>MGGEIITLQAGQCGNHVGKFLWSQLAKEHAIGTDGLSQLPDSSTERDDDTKPFFRENSRNKFTPRAIMMDSEPSVIADVENTFRGFFDPRNTWVASDGASAGNSWANGYDIGTRNQDDILNKIDKEIDSTDNFEGFQLLHSVAGGTGSGLGSNLLEALCDRYPKKILTTYSVFPARSSEVVVQSYNTILALRRLIEDSDATVVFDNASLLNISGKVFRNPNIDLQHTNQLISTIISSVTNSIRFPSYMYSSMSSIYSTLIPSPELHFLSPSFTPFTSDYIHDDIAHKGHSSYDVMLDLLDPSNSLVSTAMNNPTYFNVYNTIIGNVEPRQISRAMTKLQQRIKFPSWSSSAMHVNIGRRSPYLPLQPNENEVSGMMLSNMSTVVNVFENACNTFDKVFAKGAFLNNYNVGDLFQSMQNVQDEFAESREVVQSLMEDYVAAEQDSYLDDVLVDDENMVGELEEDLDADGDHKLV[2x];> MEIKEVDDRAELLRYTNNIPLLGKLVNHQPLWSTNPKLKSFSLEKISAPDQRRVQEALVVKDLLNVLIGLEGTYIRYFNDYEPSDPETPIEFKIAKKMDPSFKTFSRRIVRYGKQYMILTRAYEKWSDTSFGMVLQRFAYEIRRFLEDVYLKTLVERLERDFNKVPNFSIRELEQIINETEVNKQMELLYNIYEEIFREIEERRTNQSSQEDFNNFMDSMKNESSLHLRLMVAFDTTVYPVPKGGAILKIFQQKILENLGDRSSVMFLKKLLNNISQDYCTMLYEWLTQGILNDPYQEFMTYDDLEGKTDNIFDTRDRAWDTQYFIRKDVLLRDCDSEEDKNLLFKMLRTGILLKVVRASLQIPTIPSNSSDITIQEINDFADLMEGSNLELYVDKCYSRANEIFLKLFFQGYDLINVLKHLQQIFLGYQSGHNVLKFLTKNMGELTKHYRNDNNANYDKLLQNFELERQSENPNNLMRQLLMIQFDTETLPQVLSHYLQIYPEVPENNSANDDSDPLMHANNFKNMNAILFDELSKERTGAYHGSNLELYTPKSAIYHLKFDINIPYPLNIIISRTCMIKYQIILRYQLVLQYHSR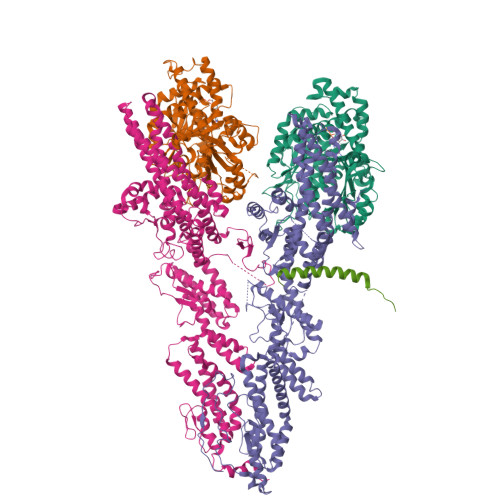LLDETWMDLNKTPSWKYRGYSHTVKRRIVRATRVLHAKMNHFIKTIMEYFNQNVIDKEVYSLEKCYRNPTLAVAIQNELEGGLTNIMTNRCLSDLIPLQLQIFDIVYKFCKFIKSMRAKLCQLDPVLYEKHKSGMMKTLNEGYRTNNGGQEDVGYQEDAALELIQKLIEYISNASSIFRKCLINFTQELSTEKFDFYDSSSVDAAGIERVLYSIVPPRSASASSQR;> MELEPTLFGIIEALAPQLLSQSHLQTFVSDVVNLLRSSTKSATQLGPLIDFYKLQSLDSPETTIMWHKIEKFLDALFGIQNTDDMVKYLSVFQSLLPSNYRAKIVQKSSGLNMENLANHEHLLSPVRAPSIYTEASFENMDRFSERRSMVSSPNRYVPSSTYSSVTLRQLSNPYYVNTIPEEDILKYVSYTLLATTSALFPFDHEQIQIPSKIPNFESGLLHLIFEAGLLYQSLGYKVEKFRMLNISPMKKALIIEISEELQNYTAFVNNLVSSGTVVSLKSLYREIYENIIRLRIYCRFTEHLEELSGDTFLIELNIFKSHGDLTIRKIATNLFNSMISLYYEYLMNWLTKGLLRATYGEFFIAENTDTNGTDDDFIYHIPIEFNQERVPAFIPKELAYKIFMIGKSYIFLEKYCKEVQWTNEFSKKYHVLYQSNSYRGISTNFFEIINDQYSEIVNHTNQILNQKFHYRDVVFALKNILLMGKSDFMDALIEKANDILATPSDSLPNYKLTRVLQEAVQLSSLRHLMNSPRNSSVINGLDARVLDLGHGSVGWDVFTLDYILYPPLSLVLNVNRPFGRKEYLRIFNFLWRFKKNNYFYQKEMLKSNDIIRSFKKIRGYNPLIRDIINKLSRISILRTQFQQFNSKMESYYLNCIIEENFKEMTRKLQRTENKSQNQFDLIRLNNGTIELNGILTPKAEVLTKSSSSKPQKHAIEKTLNIDELESVHNTFLTNILSHKLFATNTSEISVGDYSGQPYPTSLVLLLNSVYEFVKVYCNLNDIGYEIFIKMNLNDHEASNGLLGKFNTNLKEIVSQYKNFKDRLYIFRADLKNDGDEELFLLSKSLR;> MDEASHLPNGSLKNMEFTPVGFIKSKRNTTQTQVVSPTKVPNANNGDENEGPVKKRQRRSIDDTIDSTRLFSEASQFDDSFPEIKANIPPSPRSGNVDKSRKRNLIDDLKKDVPMSQPLKEQEVREHQMKKERFDRALESKLLGKRHITYANSDISNKELYINEIKSLKHEIKELRKEKNDTLNNYDTLEEETDDLKNRLQALEKELDAKNKIVNSRKVD>[2x]GHMTDRLASLFESAVSMLPMSEARSLDLFTEITNYDESACDAWIGRIRCGDTDRVTLFRAWYSRRNFGQLSGSVQISMSTLNARIAIGGLYGDITYPVTSPLAITMGFAACEAAQGNYADAMEALEAAPVAGSEHLVAWMKAVVYGAAERWTDVIDQVKSAGKWPDKF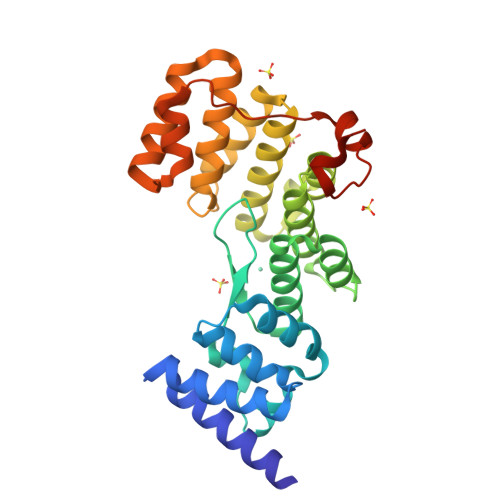LAGAAGVAHGVAAANLALFTEAERRLTEANDSPAGEACARAIAWYLAMARRSQGNESAAVALLEWLQTTHPEPKVAAALKDPSYRLKTTTAEQIASRADPWDPGSVVTDNSGRE> EKKSINECDLKGKKVLIRVDFNVPVKNGKITNDYRIRSALPTLKKVLTEGGSCVLMSHLGRPKGIPMAQAGKIRSTGGVPGFQQKATLKPVAKRLSELLLRPVTFAPDCLNAADVVSKMSPGDVVLLENVRFYKEEGSKKAKDREAMAKILASYGDVYISDAFGTAHRDSATMTGIPKILGNGAAGYLMEKEISYFAKVLGNPPRPLVAIVGGAKVSDKIQLLDNMLQRIDYLLIGGAMAYTFLKAQGYSIGKSKCEESKLEFA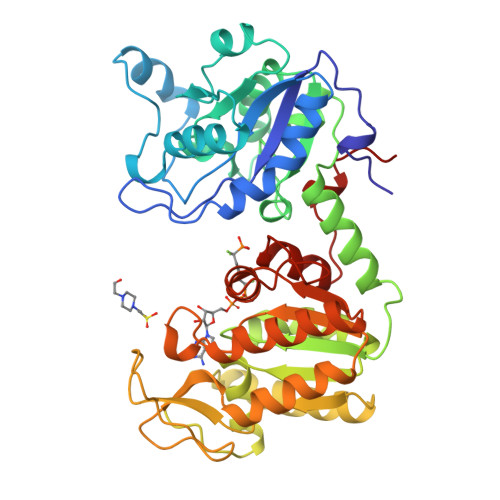RSLLKKAEDRKVQVILPIDHVCHTEFKAVDSPLITEDQNIPEGHMALDIGPKTIEKYVQTIGKCKSAIWNGPMGVFEMVPYSKGTFAIAKAMGRGTHEHGLMSIIGGGDSASAAELSGEAKRMSHVSTGGGASLELLEGKTLPGVTVLDDK> MSQQVDKIKASYPLFLDQDYKDMLAKKRDGFEEKYPQDKIDEVFQWTTTKEYQELNFQREALTVNPAKACQPLGAVLCALGFEKTMPYVHGSQGCVAYFRSYFNRHFREPVSCVSDSMTEDAAVFGGQQNMKDGLQNCKATYKPDMIAVSTTCMAEVIGDDLNAFINNSKKEGFIPDEFPVPFAHTPSFVGSHVTGWDNMFEGIARYFTLKSMDDKVVGSNKKINIVPGFETYLGNFRVIKRMLSEMGVGYSLLSDPEEVLDTPADGQFRMYAGGTTQEEMKDAPNALNTVLLQPWHLEKTKKFVEGTWKHEVPKLNIPMGLDWTDEFLMKVSEISGQPIPASLTKERGRLVDMMTDSHTWLHGKRFALWGDPDFVMGLVKFLLELGCEPVHILCHNGNERWKKAVDAILAASPYGKNATVYIGKDLWHLRS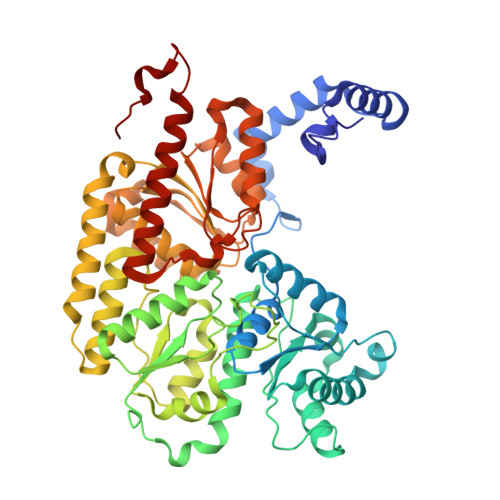LVFTDKPDFMIGNSYGKFIQRDTLHKGKEFEVPLIRIGFPIFDRHHLHRSTTLGYEGAMQILTTLVNSILERLDEETRGMQATDYNHDLVR>[2x]PPYTITYFPVRGRCEAMRMLLADQDQSWKEEVVTMETWPPLKPSCL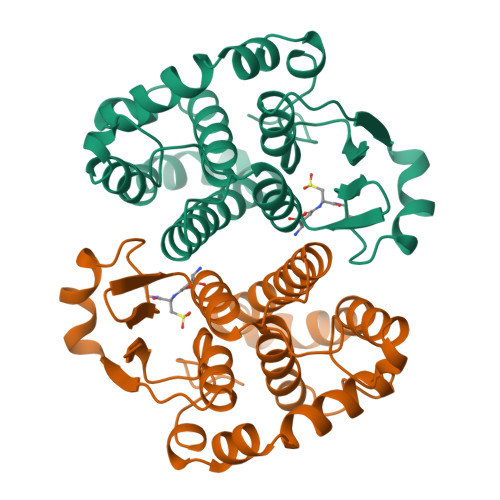FRQLPKFQDGDLTLYQSNAILRHLGRSFGLYGKDQKEAALVDMVNDGVEDLRCKYATLIYTNYEAGKEKYVKELPEHLKPFETLLSQNQGGQAFVVGSQISFADYNLLDLLRIHQVLNPSCLDAFPLLSAYVARLSARPKIKAFLASPEHVNRPINGNGKQ>[4x]SMGVRKLATIRTAGEITPIAGAEAIECCHVDGWTCVIKKGEFKQGDRGVYFEIDSFIKEDNDRYPMLSKQVIDYEGQ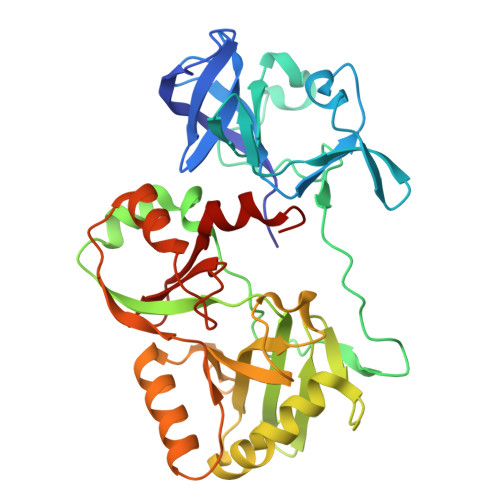RGTRLRTARLRGQLSQGLFLPMDRFPELASNQVGDDVTEILGITKWEPPISTNLSGEILGEFPTFISKTDQERVQNLIPQIEENKGQKFEVTVKLDGSSMTVYRKDDHIGVCGRNWELRETATNAQWHAARRNKMIEGLQFLNRNLALQGEIIGESIQGNLEKLKGQDFYLFDIYDIDKAQYLTPIERQSLVKQLNDNGFTVKHVPILDDLELNHTAEQILAMADGPSLNKNVKREGLVFKRLDGKFSFKAISNAYLEKHKDR>[4x]MHHHHHHMANRKLEKMASIDVHLRQLVPGKVSEDDKLVEYDALLLDRFLDILQDLHGEDLRETVQELYEHSAEYEGKHEPKKLEELGSVLTSLDPGDSIVIAKAFSHMLNLANLAEEVQIAYRRRIKKLKKGDFVDESSATTESDLEETFKKLVGDLNKSPEEIFDALKNQTVDLVLTAHPTQSVRRSLLQKHGRIRDCLAQLYAKDITPDDKQELDEA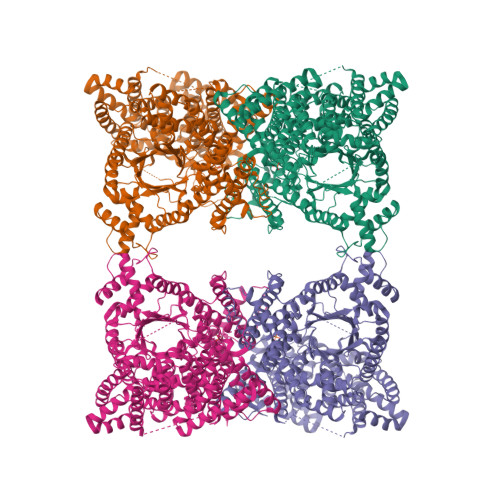LQREIQAAFRTDEIKRTPPTPQDEMRAGMSYFHETIWKGVPKFLRRVDTALKNIGIEERVPYNAPLIQFSSWMGGDRDGNPRVTPEVTRDVCLLARMMAATMYFNQIEDLMFEMSMWRCNDELRARADEVHANSRKDAAKHYIEFWKSIPTTEPYRVILGDVRDKLYHTRERAHQLLSNGHSDVPVEATFINLEQFLEPLELCYRSLCSCGDRPIADGSLLDFLRQVSTFGLSLVRLDIRQESDRHTDVLDAITTHLDIGSYREWSEERRQEWLLSELSGKRPLFGSDLPKTEEIADVLDTFHVIAELPADSFGAYIISMATAPSDVLAVELLQRECRVKQPLRVVPLFEKLADLEAAPAAVARLFSVDWYKNRINGKQEVMIGYSDSGKDAGRLSAAWQLYKAQEELVKVAKEYGVKLTMFHGRGGTVGRGGGPTHLAILSQPPDTINGSLRVTVQGEVIEQSFGEEHLCFRTLQRFTAATLEHGMRPPISPKPEWRALLDEMAVVATEEYRSVVFQEPRFVEYFRLATPELEYGRMNIGSRPSKRKPSGGIESLRAIPWIFAWTQTRFHLPVWLGFGSAIRHVIEKDVRNLHMLQDMYQHWPFFRVTIDLIEMVFAKGDPGIAALYDKLLVSEELWPFGEKLRANFEETKKLILQTAGHKDLLEGDPYLKQGLRLRDSYITTLNVCQAYTLKRIRDPSYHVTLRPHISKEIAESSKPAKELIELNPTSEYAPGLEDTLILTMKGIAAGLQNTG> WSHPQFEKMQLNKEVLKGYIDILIVSILEKKDCYGYEIAKQVRER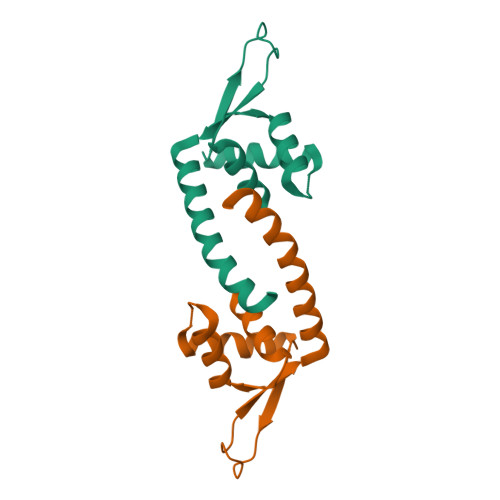SEFELKEGTMYLALKRMESKNLIKSYYSNEQSSGGRRKYYNLTNEGKDFLEIKKQEWRFIKKVMNQFLGEVD>SNAMKEPPMTKTVFHLGVTEADLNGATLAIIPGDPARVQKIAELMDNPVFLASHREYTVYRAELDGQSVVVCSTGIGGPSTSIAVEELAQLGVRTFLRVGTTGAIQPHVNVGDMIVTTGSVRLDGASLHFAPMEFPAVPDFDVATAMKAAAQESGATVHMGVTASSDTFYPGQERYDTFTGRVVRRFQGSMKEWQDMGVLNFEMESATLLTMCASSGLKAGCVAGVIINRTQKEIPDHATLKETEARSIKVVVEAARKML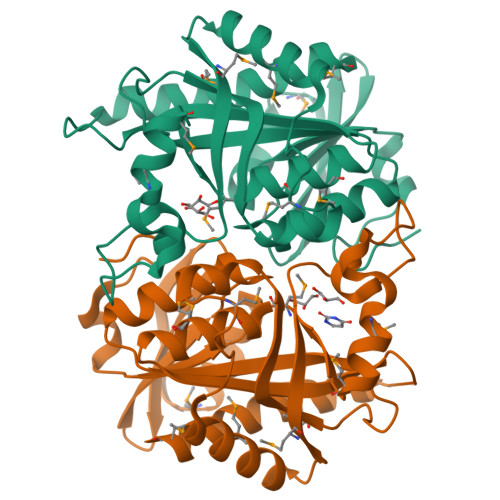K[12x]>GMLSRIDLYIKHRDIFLKHLELLHKLIEKVEDSSLNESELLNARLVDDMFPFNVQAKIATNFALRACCPLSGKEYKELEGDIDSFCGLKTYVVTAIDYINKLSEPTLEQLNLNVQDTAGFKEISMPASEYMSSFVLPNFFFHISMVY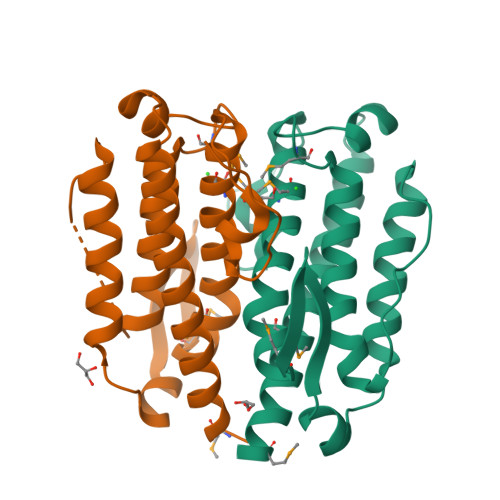AIAKNNGVSVTKGDFDGIHQYPKGFSWEA[2x]> GPDGDPGDPGDPGPDGRPGPDGP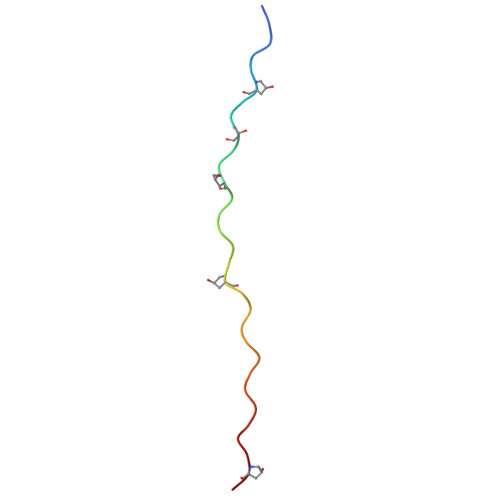DGPAGDPG>MADVTGIALGMIETRGLVPAIEAADAMTKAAEVRLVGRQFVGGGYVTVLVRGETGAVNAAVRAGADACERVGDGLVAAHIIARVHSEVENILPKAPQA[480x];>MKIMQVEKTLVSTNRIADMGHKPLLVVWEKPGAPRQVAVDAIGCIPGDWVLCVGSSAAREAAGSKSYPSDLTIIGIIDQWNGE[60x];>MPSQSGMNPADLSGLSGKELARARRAALSKQGKAAVSNKTASVNRSTKQAASSINTNQVRSSVNEVPTDYQMADQLCSTIDHADFGTESNRVRDLCRQRREALSTIGKKAAKTTGKPSGRVRPQQSVVHNDAMIENAGDTNQSSSTSLNNELSEICSIADDMPERFGSQAKTVRDICRARRQALSERGTRAVPPKPQSQGGPGRNGYQIDGYLDTALHGRDAAKRHREMLCQYGRGTAPSCKPTGRVKNSVQSGNAAPKKVETGHTLSGGSVTGTQVDRKSHVTGNEPGTCRAVTGTEYVGTEQFTSFCNTSPKPNATKVNVTTTARGRPVSGTEVSRTEKVTGNESGVCRNVTGTEYMSNEAHFSLCGTAAKPSQADKVMFGATARTHQVVSGSDEFRPSSVTGNESGAKRTITGSQYADEGLARLTINGAPAKVARTHTFAGSDVTGTEIGRSTRVTGDESGSCRSISGTEYLSNEQFQSFCDTKPQRSPFKVGQDRTNKGQSVTGNLVDRSELVTGNEPGSCSRVTGSQYGQSKICGGGVGKVRSMRTLRGTSVSGQQLDHAPKMSGDERGGCMPVTGNEYYGREHFEPFCTSTPEPEAQSTEQSLTCEGQIISGTSVDASDLVTGNEIGEQQLISGDAYVGAQQTGCLPTSPRFNQTGNVQSMGFKNTNQPEQNFAPGEVMPTDFSIQTPARSAQNRITGNDIAPSGRITGPGMLATGLITGTPEFRHAARELVGSPQPMAMAMANRNKAAQAPVVQPEVVATQEKPELVCAPRSDQMDRVSGEGKERCHITGDDWSVNKHITGTAGQWASGRNPSMRGNARVVETSAFANRNVPKPE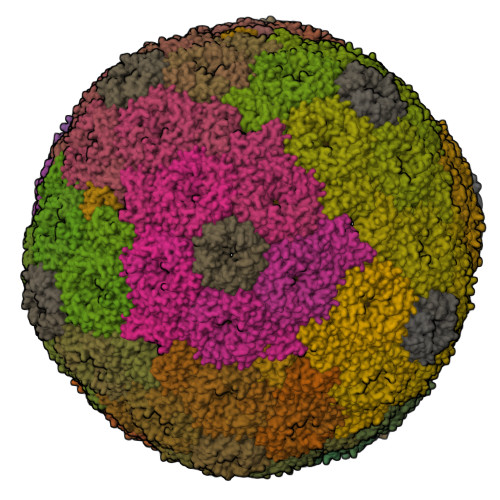KPGSKITGSSGNDTQGSLITYSGGARG[60x]Trioxacarcin A | C42 H52 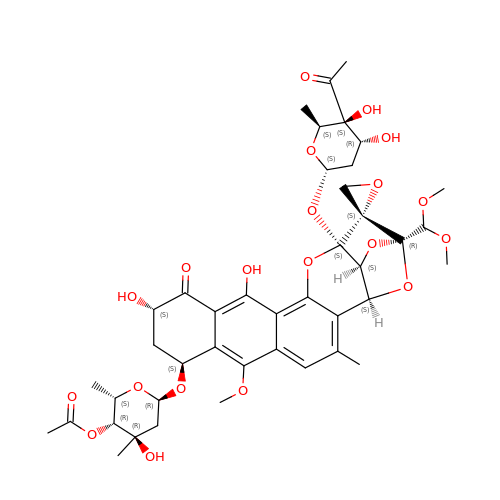O20 | VVCYZYSLUSSELI-NVJOEFDOSA-N>MLPGTFFEVLKNEGVVAIATQGEDGPHLVNTWQSYLKVLDGNRIVVPVGGMHKTEANVARDERVLMTLGSRKVAGRNGPGTGFLIRGSAAFRTD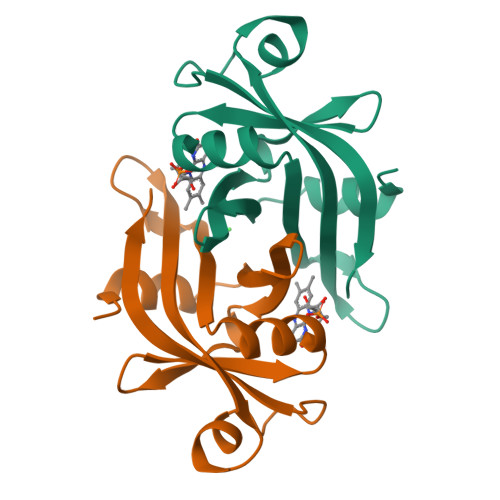GPEFEAIARFKWARAALVITVVSAEQTL[2x]>[3x]MGNRLSKIATRTGDDGTTGLGDGSRVRKDDARIAAIGDVDELNSQIGVLLAEPLPDDVRAALSAIQHDLFDLGGELCIPGHAAITDAHLARLDGWLAHYNGQLPPLEEFILPGG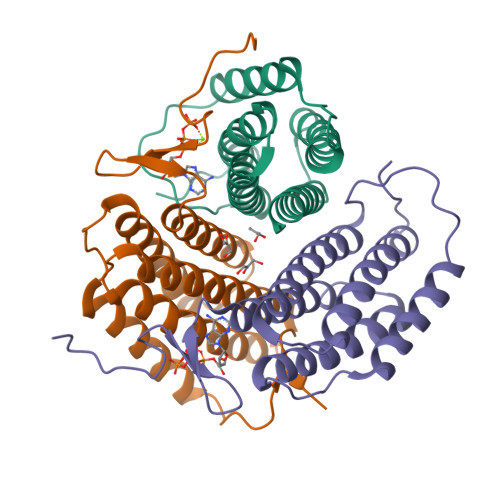ARGAALAHVCRTVCRRAERSIVALGASEPLNAAPRRYVNRLSDLLFVLARVLNRAAGGADVLWDRTRAH> VPSYDSFDYEDYPAALPNHKPKGTFKDYVRDRADLNKDKPVIPAAALAGYTGSGPIQLWQFLLELLTDKSCQSFISWTGDGWEFKLSDP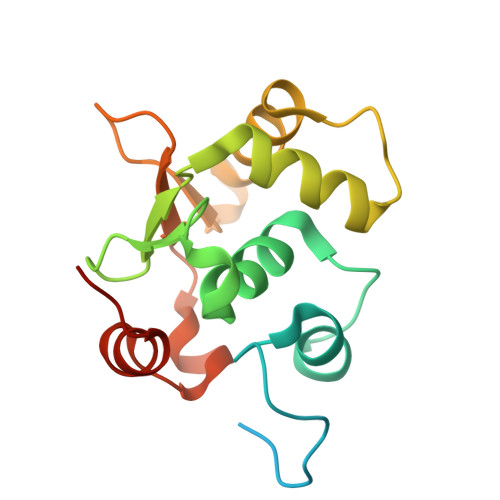DEVARRWGKRKNKPKMNYEKLSRGLRYYYDKNIIHKTAGKRYVYRFVCDLQSLLGYTPEELHAMLDVKPDAD> XEVNPAV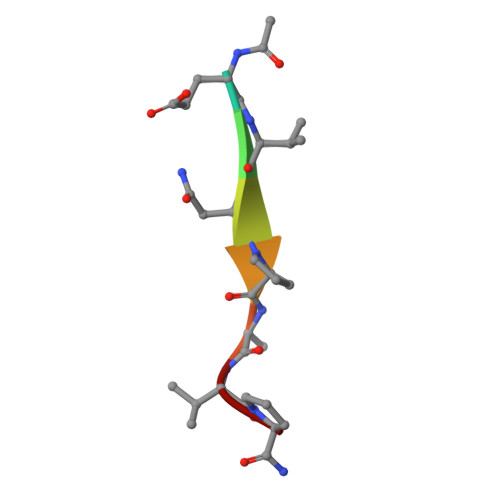P6-AMINOHEXYL-URIDINE-C1,5'-DIPHOSPHATE | C15 H27 N3 O12 P2 | 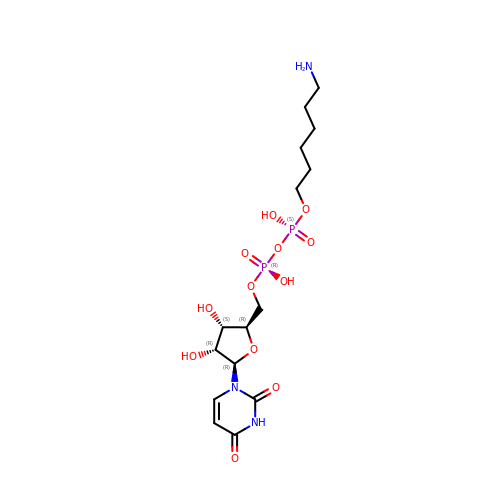MLWJBKPFDKRHBM-FMKGYKFTSA-N> DGGICPRI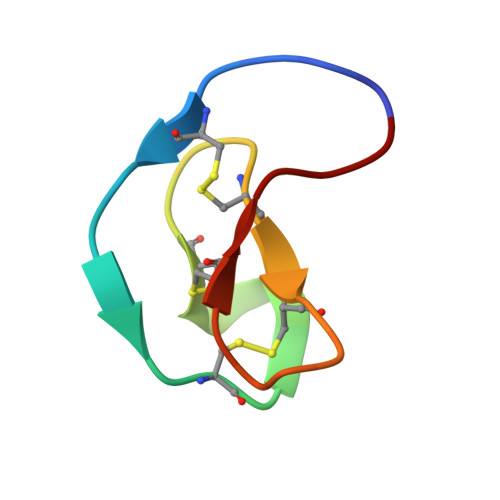GRLCRRDSDCPGACICRATRFCGSGY3-(butylamino)-4-phenoxy-5-sulfamoylbenzoic acid | C17 H20 N2 O5 S | 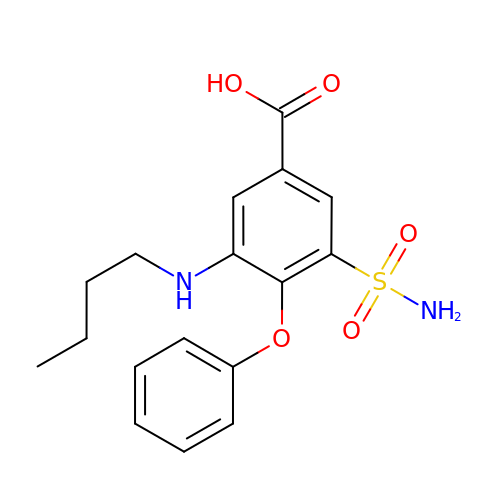MAEIEVLCKWDQJH-UHFFFAOYSA-N>[4x]MSLPIDEHVNAVKTVVVPAAGLGTRFLPATKTVPKELLPVVDTPGIELIAAEAAELGATRLAIITAPNKAGVLAHFERSSELEETLMERGKTDQVEIIRRAADLIKAVPVTQDKPLGLGHAVGLAESVLDDDEDVVAVMLPDDLVLPTGVMERMAQVRAEFGGSVLCA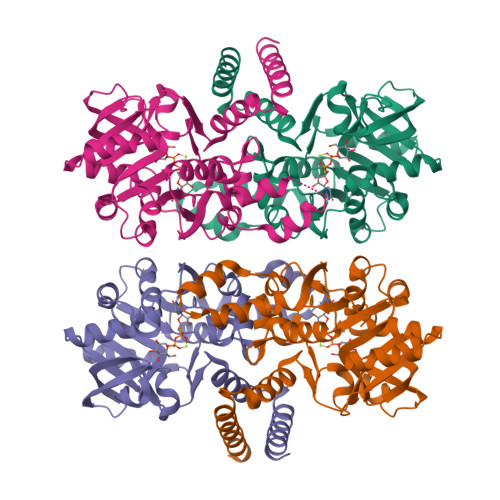VEVSEADVSKYGIFEIEADTKDSDVKKVKGMVEKPAIEDAPSRLAATGRYLLDRKIFDALRRITPGAGGELQLTDAIDLLIDEGHPVHIVIHQGKRHDLGNPGGYIPACVDFGLSHPVYGAQLKDAIKQILAEHEAAERIADDSQVKLEHHHHHH>MEGPAGYLR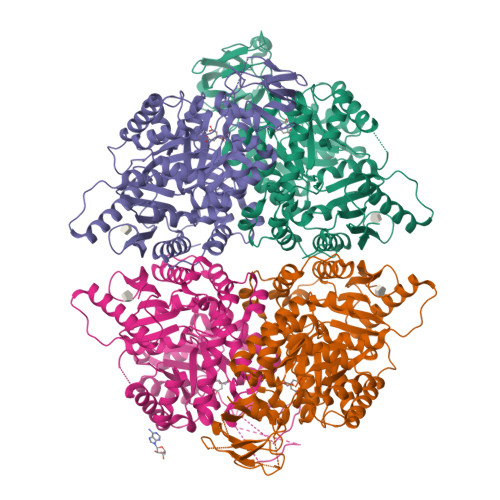RASVAQLTQELGTAFFQQQQLPAAMADTFLEHLCLLDIDSEPVAARSTSIIATIGPASRSVERLKEMIKAGMNIARLNFSHGSHEYHAESIANVREAVESFAGSPLSYRPVAIALDTKGPEIRTGILQGGPESEVELVKGSQVLVTVDPAFRTRGNANTVWVDYPNIVRVVPVGGRIYIDDGLISLVVQKIGPEGLVTQVENGGVLGSRKGVNLPGAQVDLPGLSEQDVRDLRFGVEHGVDIVFASFVRKASDVAAVRAALGPEGHGIKIISKIENHEGVKRFDEILEVSDGIMVARGDLGIEIPAEKVFLAQKMMIGRCNLAGKPVVCATQMLESMITKARPTRAETSDVANAVLDGADCIMLSGETAKGNFPVEAVKMQHAIAREAEAAVYHRQLFEELRRAAPLSRDPTEVTAIGAVEAAFKCMAAAIIVLTTTGRSAQLLSRYRPRAAVIAVTRSAQAARQVHLCRGVFPLLYREPPEAIWADDVDRRVQFGIESGKLRGFLRVGDLVIVVTGWRPGSGYTNIMRVLSIS[4x]>[2x]GTGIKVFFVTPEGREIMIEGNEGDSILDLAHANNIDLEGACE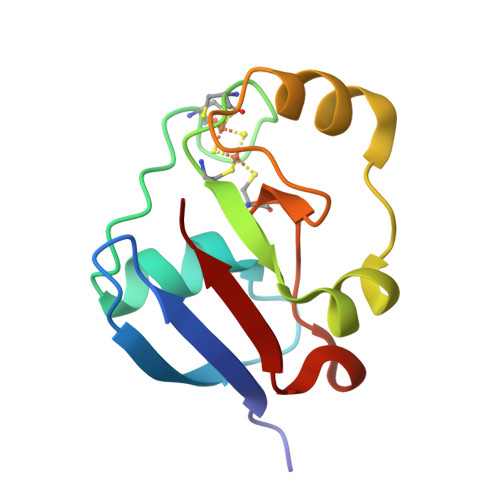GSVACSTCHVIVDPEHYELLDPPEEDEEDMLDLAFGLEETSRLGCQVLLRKDLDGIRVRIP>[2x]HMNFKMEHQNKRSPLHAAAEAGHVD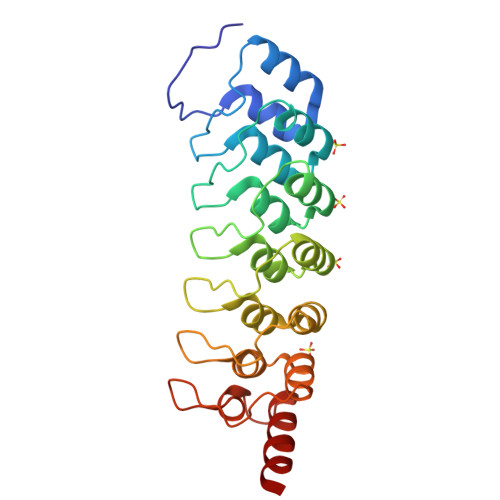ICHMLVQAGANIDTCSEDQRTPLMEAAENNHLEAVKYLIKAGALVDPKDAEGSTCLHLAAKKGHYEVVQYLLSNGQMDVNCQDDGGWTPMIWATEYKHVDLVKLLLSKGSDINIRDNEENICLHWAAFSGCVDIAEILLAAKCDLHAVNIHGDSPLHIAARENRYDCVVLFLSRDSDVTLKNKEGETPLQCASLNSQVWSALQMSKALQDSA> QGMKTRLEQVLERYLNGREVAVWGVPTRRLLRALKPFKFHTADRVDPQYHYVVAVTDDDLTDFLSDEQSKSFQYANDYLTFDDEGGELPFERMCFNVPVGRQTYFGDGVVGACENGYIKSIGQFTSINGTAEIHANHQLNMTFVSDDIQNFFNEESMAVFQEKLRKDPKHPYAYSKEPMTIGSDVYIGAHAFINASTVTSIGDGAIIG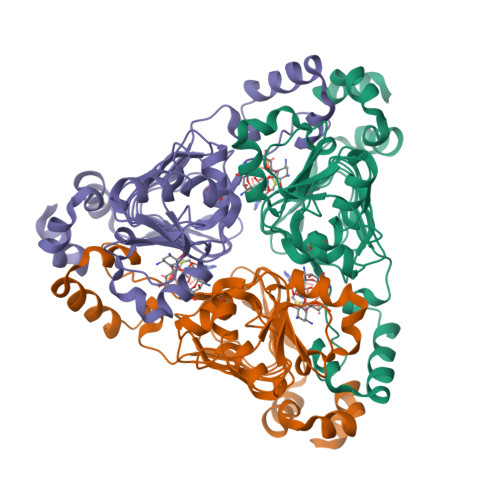SGAVVLENVPPFAVVVGVPARIKRYRFSKEMIETLLRVKWWDWSIEEINENVDALISPELFMKKYGSL>NUGUACA[2x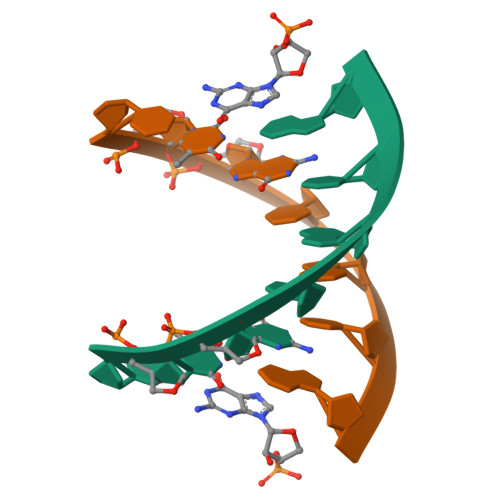]> RRRRRSLDASSDSLSGSDMEVDSDGESIDAPLPLDSFLRDANSFKVAAEDSARSAKRRKLRPETIDIQRTRDIPDTHKAAISSLAFHPRYPILLSSSTSSIMYLHKLDASAYPTPNPLLTSVHVKRTDLRRAAFVGPDGGEIIFAGRRRYF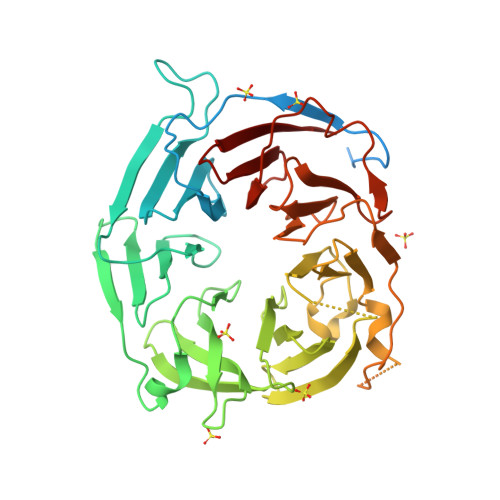HCWNLSSGLVKKVSKIQGHQKEQRTMERFRVSPCGRYMALVASDKKGGGMLNIINVGTMQWIAQARIDGRHGVADFAWWSDGNGLTIAGRDGQVTEWSMITRRTVGIWRDEGSIGGTVMALGGRNGPAELGGDRWVAIGSNSGILNVYDRNDLIEKPPKKNESNQEEQNSSEKTKEIRIKKYPTPTRVFEQLTTSISVVAFSPDGQLLAFGSQHKKDALRLVHLPSCTVYRNWPTEQTPLGRVTAIAFSSKSDVLAVGNDVGRVRLWEIRG> GSINMATVPVYCVCRLPYDVTRFMIECDACKDWFHGSCVGVEEEEAPDIDIYHCPN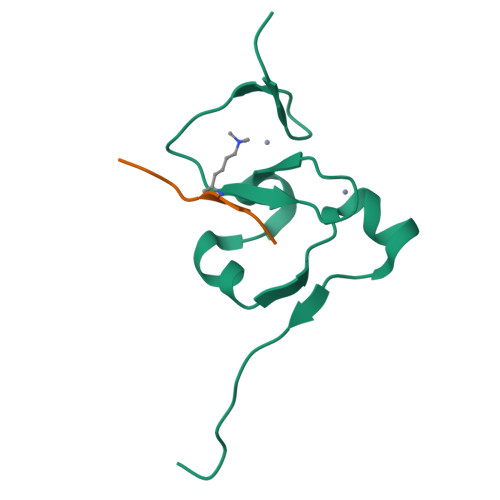CEKTHGKSTLKKKRTWHK;> PRVKAAQAGRQS> GSHMEMAGDLSAGFFMEELNTYRQKQGVVLKYQELPNSGPPHDRRFTFQVIIDGREFPEGEGRSKKEAKNAAAKLAVEILNKEKKAVSPLLLTTTNSSEGLSMGNYIGLINRIAQKKRLTVNYEQCASGVHGPEGFHYKCKMGQKEYSIGTGSTKQE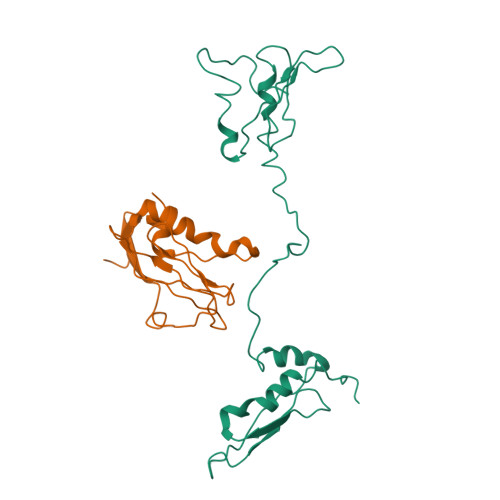AKQLAAKLAYLQILSEETGSGC;> TPASRYITDMTIEELSRDWFMLMPKQKVEGPLCIRIDQAIMDKNIMLKANFSVIFDRLETLILLRAFTEEGAIVGEISPLPSFPGHTIEDVKNAIGVLIGGLEWNDNTVRVSKTLQRFAWGS> GPLGSTSSTSQADKEIQKMLDEYEQAIKRAQENIKKGEELEKKLDKLERQGKDLEDKYKTYEENLEGFEKLLTDSEELSLSEINEKMKAFSKDSEKLTQLMEKHKGDEKTVQSLQREHHDIKAKLANLQVLHDAHTGKKSYVNEKGNPVSSLKDAHLAINKDQEVVEHKGQFYLLQKGQWDAIKNDPAALEKAQKDYSQSKHDLATIKMEALIHKLSLEMEKQLETINDLIMSTDPKENEEATKLLHKHNGLNLKLANLQDM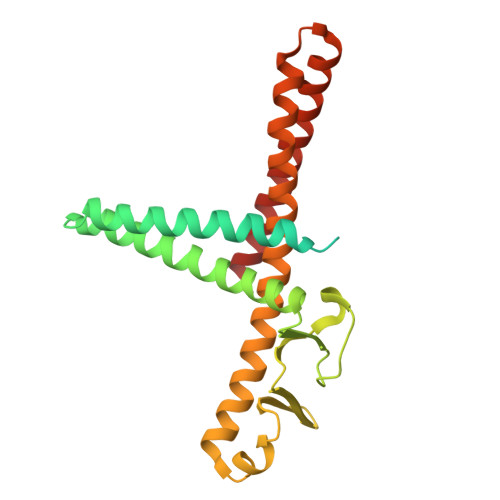LAVHR>MIRFFKIVTPILLSISLVACSSASGKTEKITAPIEKDRNLSMVVTTDVHYFAPSLTDNGKAFEKYVAAGDGKQLAYSDEITDAFLADVESKKTDVLIISGDLTNNGEKTSHEELAKKLTQVEKNGTQVFVVPGNHDINNPWARKFEKDKQLPTDTISPTDFSKIYSDFGYEDAISSDEFSLSYLAAPSSKVWLLMLDTAIYKTNMQQGNPTTEGGLTAGTLDWIKESSALAKKNGAKLIPVLHHNLTDHNDVIQKGYTINYNQQVIDALTEGAMDFSLSGHIHTQNIRSAKSTDGKEITDIVTNALSVFPHKYGNITYSAKNKNFTYQSQKLDMEAWAKAQGSTDENLLNFDQFDYETFYNSGYDKAMMDLMTDESYDKYNQADKEKMADTMGLNNMYFFAGTAPPKSD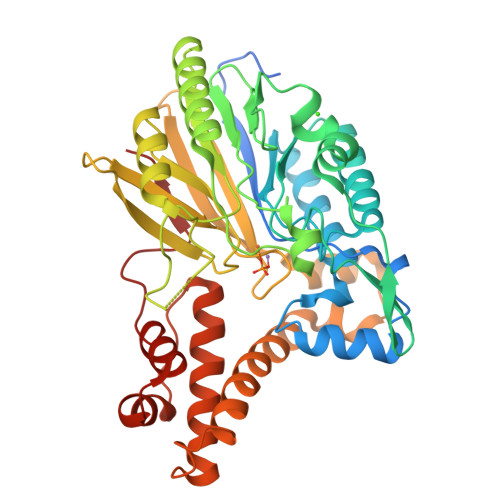GMALWDSAPNSFLKDYVLSSSNPPKKSNDYYVSP[2x]propan-2-yl ~{N}-[(2~{S},4~{R})-1-ethanoyl-6-(furan-2-yl)-2-methyl-3,4-dihydro-2~{H}-quinolin-4-yl]carbamate | 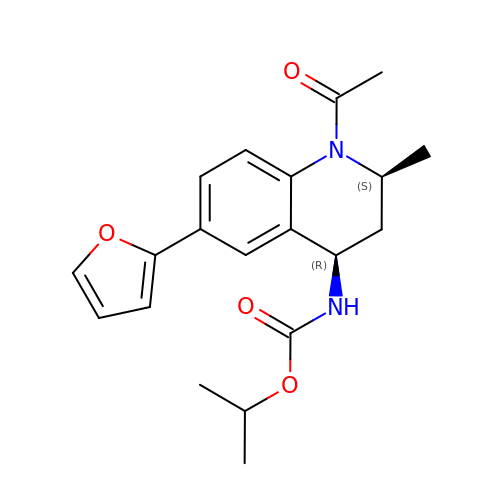C20 H24 N2 O4 | OZBRAEGGHPSXJE-SUMWQHHRSA-N> GSLKIKTIGDRCLRQKSEEVEFDKKEMSELYDQMCEAMWASDGIGLAAPQV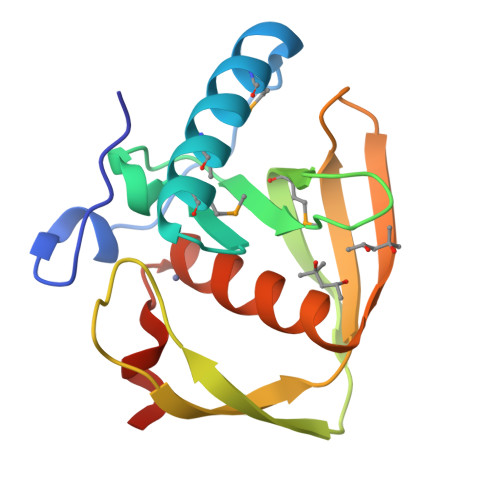GINKRVIVVDETTEEHGKYAHLMVNPKITWKSEEKVLFDEGCLSVPDQNGEVLRPKSIKVTFQNKDGKYKKWKLDGLAARVVQHEIDHLEGILFVDYFNDKEN(2S,4R)-1-[(3-chloro-2-fluorophenyl)methyl]-2-methyl-4-({3-[(1,3-thiazol-2-yl)amino]isoquinolin-1-yl}methyl)piperidine-4-carboxylic acid | C27 H26 Cl F N4 O2 S | 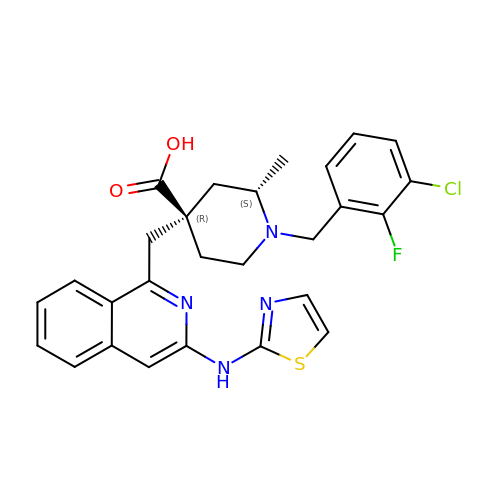GKVNGMCPNCGMBE-CBZJRKILSA-N>[2x]HCVILNDGNFIPVLGFGTALPLECPKSKAKELTKIAIDAGFHHFDSASVYNTEDHVGEAIRSKIADGTVRREDIFYTSKVWCTSLHPELVRASLERSLQKLQFDYVDLYLIHYPMALKPGEENFPVDEHGKLIFDRVDLCATWEAMEKCKDAGLTKSIGVSNFNY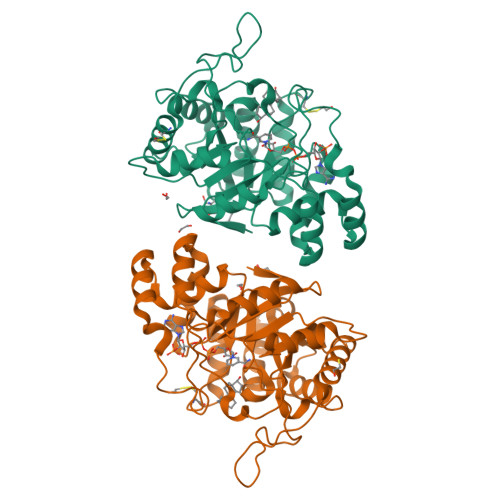RQLEMILNKPGLKYKPVCNQVECHPYLNQMKLLDFCKSKDIVLVAYGVLGTQRYGGWVDQNSPVLLDEPVLGSMAKKYNRTPALIALRYQLQRGIVVLNTSLKEERIKENMQVFEFQLSSEDMKVLDGLNRNMRYIPAAIFKGHPNWPFLDEY>[12x]MHHHHHHMVIGLSTGSDDDDVEVIGGVDPRLIAVQENDSDESSLTDLVEQPAKVMRIGTMIKQLLEEVRAAPLDEASRNRLRDIHATSI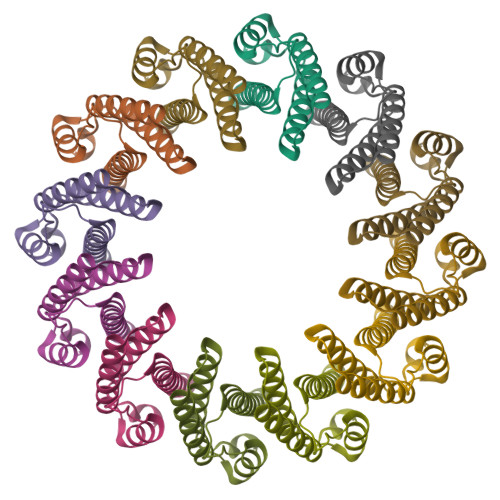RELEDGLAPELREELDRLTLPFNEDAVPSDAELRIAQAQLVGWLEGLFHGIQTALFAQQMAARAQLQQMRQGALPPGVGKSGQHGHGTGQYL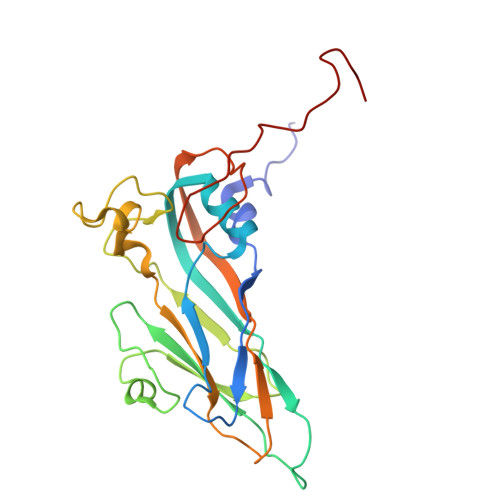> NYHSRSESTVENFLCRSACVFYTTYRNHGTDGDNFGYWVINTRQVAQLRRKLEMFTYARFDLELTFVITSTQEQSTIQGQDSPVLTHQIMYVPPGGPVPTKVNSYSWQTSTNPSVFWTEGSAPPRMSIPFISIGNAYSMFYDGWAKFDKQGTYGINTLNNMGTLYMRHVNDGSPGPIVSTVRIYFKPKHVKTWVPRPPRLCQYQKAGNVNFEPTGVTESRTDITTMQ>[2x]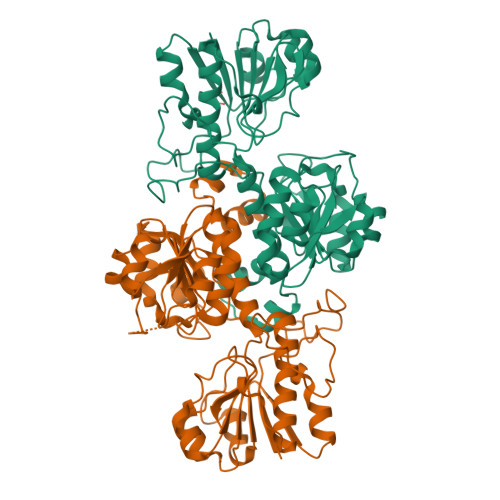MAKVLCVLYDDPVDGYPKTYARDDLPKIDHYPGGQTLPTPKAIDFTPGQLLGSVSGELGLRKYLESNGHTLVVTSDKDGPDSVFERELVDADVVISQPFWPAYLTPERIAKAKNLKLALTAGIGSDHVDLQSAIDRNVTVAEVTYCNSISVAEHVVMMILSLVRNYLPSHEWARKGGWNIADCVSHAYDLEAMHVGTIAAGRIGLAVLRRLAPFDVHLHYTDRHRLPESVEKELNLTWHATREDMYPVCDVVTLNIPLHSPTEHMINDETLKLFKRGAYIVNTARGKLCDRDAVARALESGRLAGYAGDVWFPQPAPKDHPWRTMPYNGMTPHISGTTLTAQARYAAGTREILECFFEGRPIRDEYLIVQGGALAGTGAHNYFKGNATGGSEEAAKFKKAV2-(2-methylprop-2-enoxyamino)-2-oxidanylidene-ethanoic acid | C6 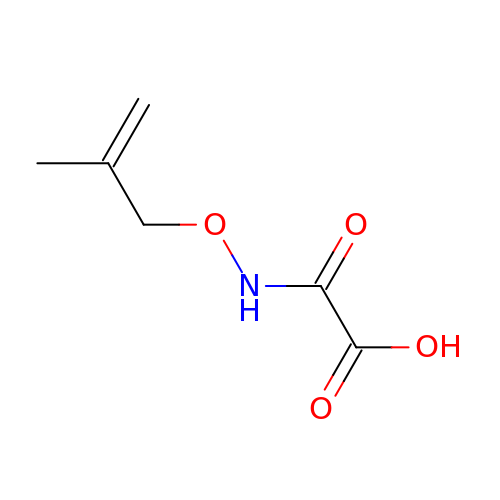H9 N O4 | GDURBQSLKIXQCN-UHFFFAOYSA-N>[4x]NIMSSAFYQQIQQQIEEVKAEGLYKSER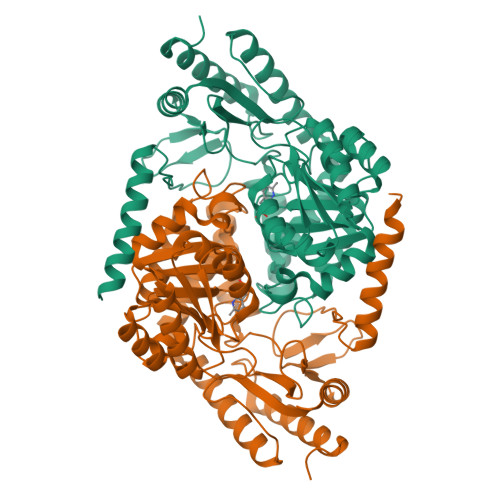IITSQQQAAVKIASGEEVLNFCANNYLGLANHPALIEAGKAGMDEHGFGMASVRFICGTQDIHKELEQKLSTFLGKEDTILYTSCFDANAGLFETILDKEDAIISDALNHASIIDGVRLCKAMRFRYSNNNMTELEEQLIAAKDAGARNILIVTDGVFSMDGVVANLPAICDLAEKYGALTMVDDSHAVGFMGKTGAGTHEYHDVVDRIDIITGTLGKAMGGASGGYTSGKKEVIEWLRQRSRPYLFSNSVAPAIVSASIRVLDLLQESGDLRDRLWENATHFRTRMSEAGFTLAGADHAIIPIMLGDAKVAAEFAERALEKGIYVIGFSFPVVPKGQARIRTQMSAAHSREQLDKAIDAFIEVGRDMEIIK>[3x]GSHMTVPTWQVRDLRRILRVSELRQHLRQARTDFRSTLSQFVYFNRSVVNPNAYDDEYLLSDQRLTYVYVDEVTAQL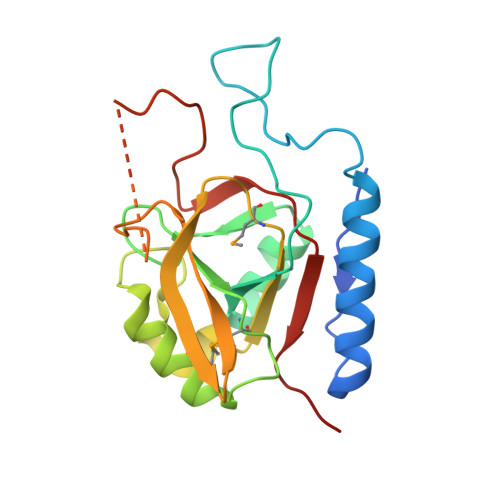CGLNRLLPSNSPAFGTVATAMPPWLLDPQEMNAILQQSCGQGGFVNYHHGPSTNSFFLAILMSQLFIRIRTDVIRGQGYGWYARLGNYVEEGEDNEGIENEEEEEEEEEETREFQLSDLIHYPIVALGSCHLTR>[4x]ARLANFL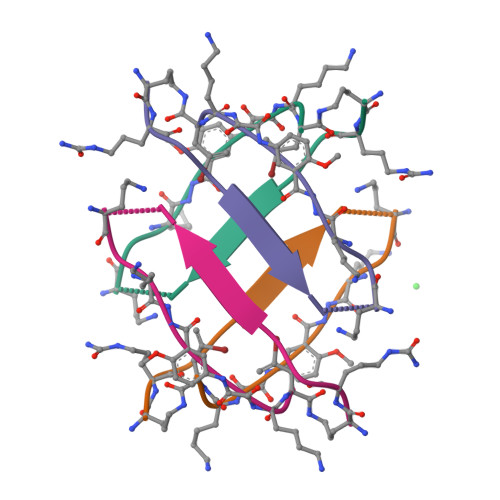VAIKXKX> MHHHHHHMVHITLDRNTANSWLIISKDRRQVRMGDTHQNVSDNKERFSNYPMVLGAQRFSSGKMYWEVDVTQKEAWDLGVCRDSVQRKGQFSLSPENGFWTIWLWQDSYEAGTSPQTTLHIQVPPCQIGIFVDYEAGVVSFYNITDHGSLIYTFSECVFAGPLRPFFNVGFNYSGGNAAPLKLCPLKM

TRIM21 plays a crucial role in immune defence, acting as an E3 ubiquitin ligase that facilitates the ubiquitination and degradation of target proteins via the proteasome pathway. TRIM21 has a unique position within the TRIM family due to its ability to specifically bind to the Fc region of intracellular antibodies, resulting in the degradation of antibody-coated proteins or of non-enveloped viral particles.

To further investigate the binding mechanism, mouse TRIM21 was used as a structural surrogate due to its improved protein stability and high sequence similarity to the human counterpart. To understand its mode of binding, we solved the high-resolution crystal structure of the murine TRIM21 PRYSPRY domain in complex with suramin at 1.3 Å resolution. Interestingly, TRIM21 residues located within 5 Å of the suramin binding site are highly conserved between the human and mouse orthologues, even though the suramin binding site is located far from the substrate binding site. The only species-specific difference within this binding site is the substitution of lysine (Lys464) in the mouse protein with threonine in the human protein. Overall, the compound binding induced minimal structural changes, with only slight adjustments of side chains in the surrounding residues compared with the apo structure. A notable exception is the outward movement of the C-terminal region (Cys466 and Pro467) to form a pocket that was completely occupied by a tolyl moiety of suramin.> NPVERYVDEVLNEVLVVPNINQSHPTTSNAAPVLDAAETGHTNKIQPEDTIETRYVQSSQTLDEMSVESFLGRSGCIHESVLDIVDNYNDQSFTKWNINLQEMAQIRRKFEMFTYARFDSEITMVPSVAAKDGHIGHIVMQYMYVPPGAPIPTTRDDYAWQSGTNASVFWQHGQPFPRFSLPFLSIASAYYMFYDGYDGDTYKSRYGTVVTNDMGTLCSRIVTSEQLHKVKVVTRIYHKAKHTKAWCPRPPRAVQYSHTHTTNYKLSSEVHNDVAIRPRTNLTTV;> SPSVEACGYSDRIIQITRGDSTITSQDVANAVVGYGVWPHYLTPQDATAIDKPTQPDTSSNRFYTLDSKMWNSTSKGWWWKLPDALKDMGIFGENMFYHFLGRSGYTVHVQCNASKFHQGTLLVVMIPEHQLATVNKGNVNAGYKYTHPGEAGREVGTQVENEKQPSDDNWLNFDGTLLGNLLIFPHQFINLRSNNSATLIVPYVNAVPMDSMVRHNNWSLVIIPVCQLQSNNISNIVPITVSISPMC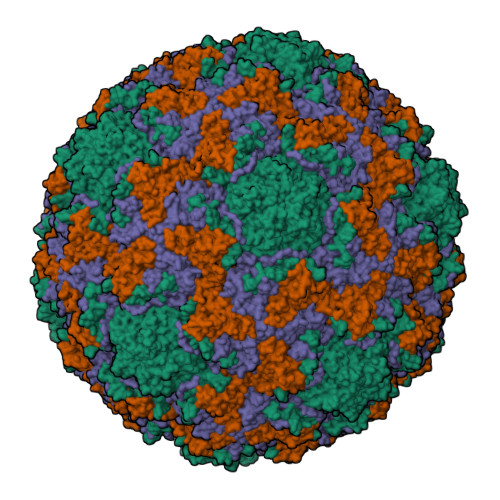AEFSGARAKTVVQ;> GLPVYVTPGSGQFMTTDDMQSPCALPWYHPTKEIFIPGEVKNLIEMCQVDTLIPINSTQSNIGNVSMYTVTLSPQTKLAEEIFAIKVDIASHPLATTLIGEIASYFTHWTGSLRFSFMFCGTANTTLKVLLAYTPPGIGKPRSRKEAMLGTHVVWDVGLQSTVSLVVPWISASQYRFTTPDTYSSAGYITCWYQTNFVVPPNTPNTAEMLCFVSGCKDFCLRMARDTDLHKQTGPITQ;> GAQVSRQNVGTHSTQNMVSNGSSLNYFNINYFKDAASSGASRLDFSQDPSKFTDPVKDVLEKGIPTLQ> SGGNPGERLRKKKWDLSELPKFEKNFYVEHPEVARLTPYEVDELRRKKEITVRGGDVCPKPVFAFHHANFPQYVMDVLMDQHFTEPTPIQCQGFPLALSGRDMVGIAQTGSGKTLAYLLPAIVHINHQPYLERGD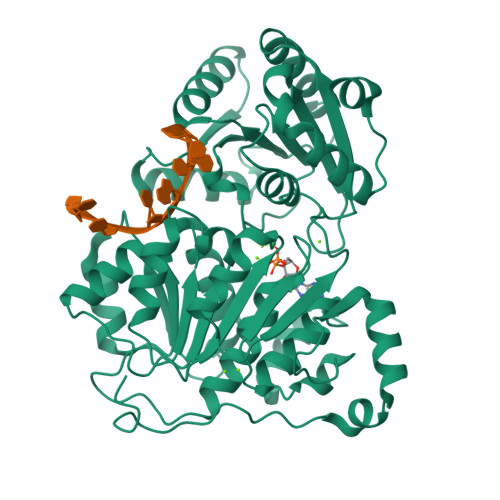GPICLVLAPTRELAQQVQQVADDYGKCSRLKSTCIYGGAPKGPQIRDLERGVEICIATPGRLIDFLESGKTNLRRCTYLVLDEADRMLDMGFEPQIRKIVDQIRPDRQTLMWSATWPKEVRQLAEDFLRDYTQINVGNLELSANHNILQIVDVCMESEKDHKLIQLMEEIMAEKENKTIIFVETKRRCDDLTRRMRRDGWPAMCIHGDKSQPERDWVLNEFRSGKAPILIATDVASRGLDVEDVKFVINYDYPNSSEDYVHRIGRTARSTNKGTAYTFFTPGNLKQARELIKVLEEANQAINPKLMQLVDHRG> SKPRNQNQVMPYQNVPGWGYSLYKGIDMSVPLAYDPNNELGDLRDVFPSAVDEMAIGYVCGNPAIKHVLTWSTTDVVQNPISNGDDWGGVIPVG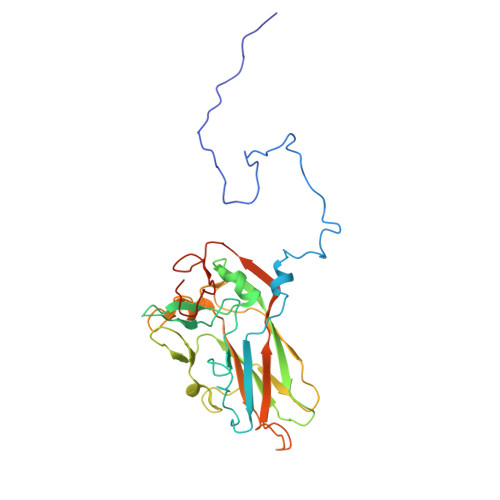MPCYSKTIRAVKGATSTSKTEVMDPAPCEYVANLFSYWRATMCYRITVVKTAFHTGRLEIFFEPGSIPTVRTADNLGPDQTQLNGTIAPSDNNYKYILDLTNDTEVTIKVPYVSNKMFMKTVGIYGAHDEDNWNFDESFTGFLCIRPITKLMAPDTVSQKVSIVVWKWAEDVVVVEPKPLTSGPTQVYNPPAVARDLVKQIDVSMQ5'-O-{[(1R)-1-hydroxydodecyl]sulfamoyl}adenosine | C22 H38 N6 O7 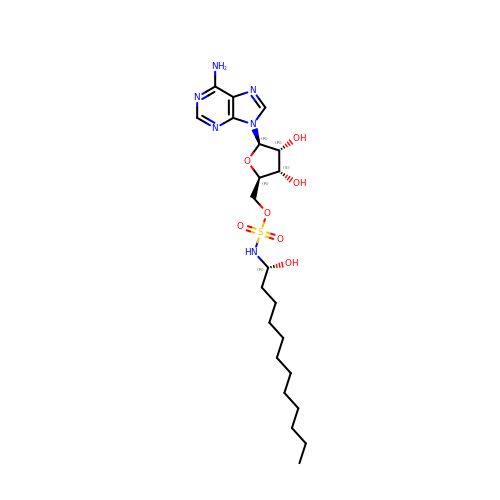S | MDBNEGOGGFLHNH-FBLYDNEXSA-N>[2x]AEPVYPDQLRLFSLGQGVCGDKYRPVNREEAQSVKSNIVGMMGQWQISGLANGWVIMGPG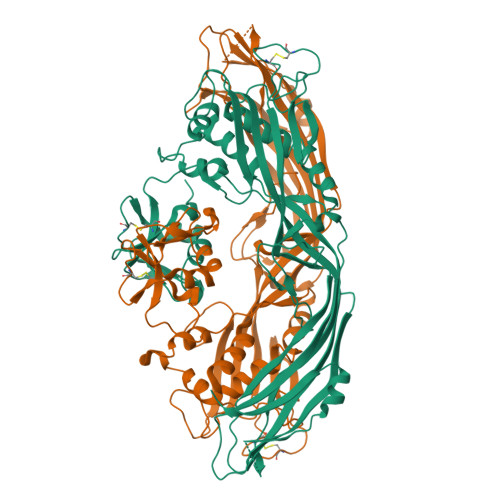YNGEIKPGTASNTWCYPTNPVTGEIPTLSALDIPDGDEVDVQWRLVHDSANFIKPTSYLAHYLGYAWVGGNHSQYVGEDMDVTRDGDGWVIRGNNDGGCDGYRCGDKTAIKVSNFAYNLDPDSFKHGDVTQSDRQLVKTVVGWAVNDSDTPQSGYDVTLRGDTATNWSKTNTYGLSEKVTTKNKFKWPLVGETELSIEIAANQSWASQNGGSTTTSLSQSVRPTVPARSKIPVKIELYKADISYPYEFKADVSYDLTLSGFLRWGGNAWYTHPDNRPNWNHTFVIGPYKDKASSIRYQWDKRYIPGEVKWWDWNWTIQQNGLSTMQNNLARVLRPVRAGITGDFSAESQFAGNIEIGAPVPLAADSKVRRARSVDGAGQGLRLEIPLDAQELSGLGFNNVSLSVTPAANQ>[2x]GSFDLEDVQPNKTTGVSKEEYKDVETDKKVKEQLGELMEPALGYVVKVPVSQSGVKRTEISNPEAITDEDLNKIPNYEIIKGVAYPNYGELVDKTAAETMKYVRSGYVIDVYHSGTRDKGYVFYKGITPSKELPQGPALTYQGEWDFTSDANLNNEEGRPTALNDDYYTTAIGKRAGLVSGDAKPSKHKYTSQFKVDFATKKMTGKLSDKEKTIYTVNADIRGNRFTGSATASDKDKGKGASYNFFSVDSQSLEGGFYGPKAEEMAGKFVADDKSLFAVFSAKHNASNVNTVRIIDASKIDLTNFSISELTNFGDASVLIIDGKKMELAGSEFTNKHTIDINGKKMVAVACCSNLEYMKFGQLWQQTEGEKQVKDNSLFLQGERTATDKMPKDGNYKYIGTWDAQVSKENNYWVATADDDRKAGYRTEFDVDFGSKNLSGKLFDKNGVNPVFTVNAKIDGNGFTGEAKTSDAGFVLDPGSLRHDNVKFSDVAVS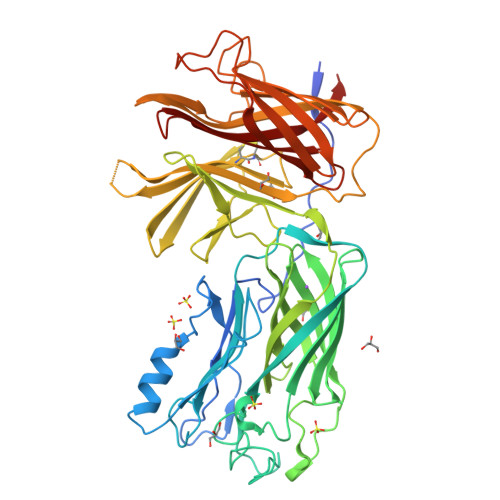GGFYGPTAAELGGQFRYQSDNGSVGVGAVFGAKQQVKK>GSSGSSGMTQFWLWVGFIGMVIGCIYFGMKASAMRRREGMEFPLESFFITLWAAALYLTMILGETVTPINGQTVFWGRYIDWVVTTPLLLMELGVIAGLRPKLIAGVMGADIFMIVTGFIGAVEAPPYNYLWWLISTGSFLAILGSLLTEYSASAKRRNGRINSLFQTLRNILIVLWICYPIVWILGAEGFHVISVGWETLCY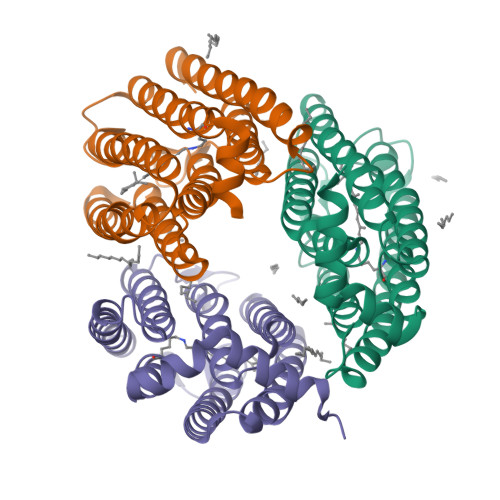SVLDVCAKVGFGFVVVSAGNETLAQASNSDRIMETVHSYMQSEEREQSPYR[3x]[1,1'-biphenyl]-3,4'-dicarboxylic acid | C14 H10 O4 | 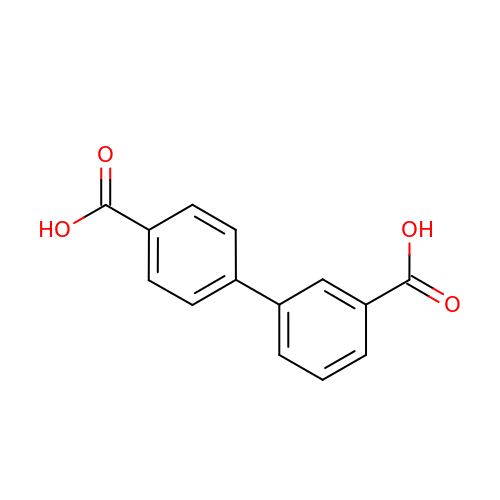GSYIVQLTSZFJRV-UHFFFAOYSA-N> QHRSRSESSIESFFARGACVTIMTVDNPASTTNKDKLFAVWKITYKDTVQLRRKLEFFTYSRFDMELTFVVTANFTETNNGHALNQVYQIMYVPPGAPVPEKWDDYTWQTSSNPSIFYTYGTAPARISVPYVGISNAYSH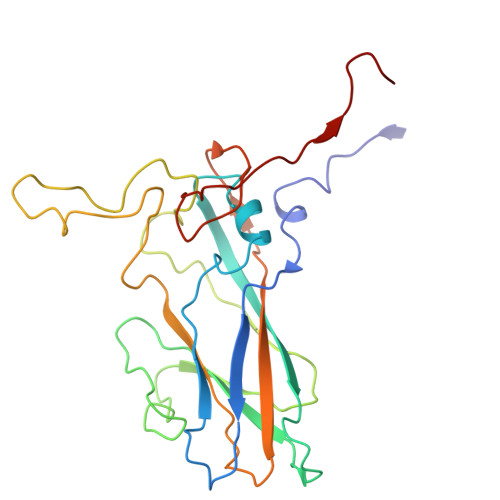FYDGFSKVPLKDQSAALGDSLYGAASLNDFGILAVRVVNDHNPTKVTSKIRVYLKPKHIRVWCPRPPRAVAYYGPGVDYKDGTLTPLSTKDLTTY> KV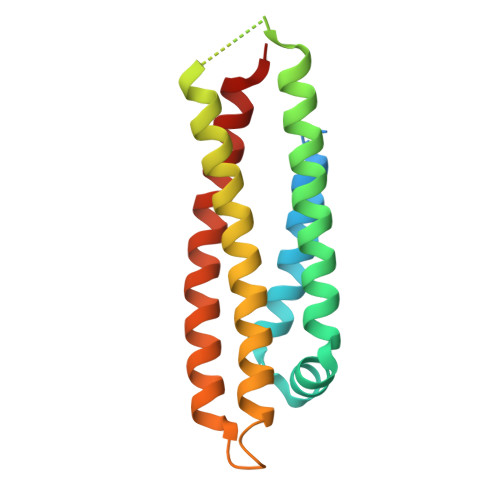EQAVETEPEPELRQQTEWQSGQRWELALGRFWDYLRWVQTLSEQVQEELLSSQVTQELRALMDETMKELKAYKSELEEQLTPVAEETRARLSKELQAAQARLGADMEDVCGRLVQYRGEVQAMLGQSTEELRVRLASHLRKLRKRLLRDADDLQKRLAVYQAG> MIFLAILDLKSLVLNAINYWGPKNNNGIQGGDFGYPISEKQIDTSIITSTHPRLIPHDLTIPQNLETIFTTTQVLTNNTDLQQSQTVSFAKKTTTTTSTSTTNGWTEGGKISDTLEEKVSVSIPFIGEGGGKNSTTIEANFAHNSSTTTFQQASTDIEWNISQPVLVPPRKQVVATLVIMGGNFTIPMDLMTTIDSTEHYSGYPILTWISSPDNSYNGPFMSWYFANWPNLPSGFGPLNSDNTVTYTGSVVSQVSAGVYATVRFDQ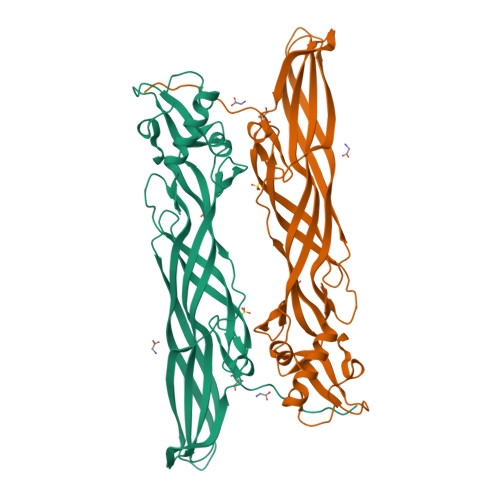YDIHNLRTIEKTWYARHATLHNGKKISINNVTEMAPTSPIKTN>SPMAMTERLKVMTIFGTRPEAIKMAPLVLELQKHPEKIESIVTVTAQHRQMLDQVLSIFGITPDFDLNIMKDRQTLIDITTRGLEGLDKVMKEAKPDIVLVHGDTTTTFIASLAAFYNQIPVGHVEAGLRTWDKYSPYPEEMNRQLTGVMADLHFSPTAKSATNLQKENKDESRIFITGNTAIDALKTTVKETYSHPVLEKLGNNRLVLMTAHRRENLGEPMRNMFRAIKRLVDKHEDVQVVYPVHMNPVVRETANDILGDYGRIHLIEPLDVIDFHNVAAR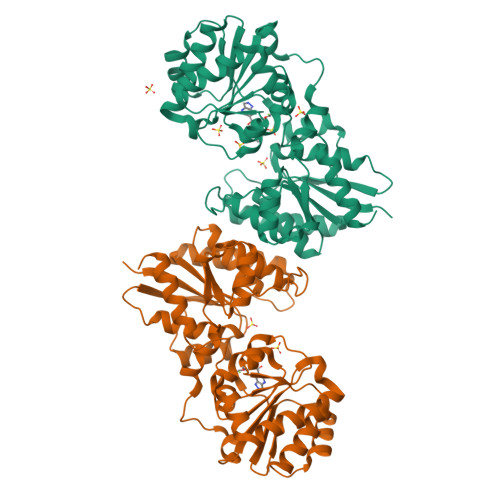SYLMLTDSGGVQEEAPSLGVPVLVLRDTTERPEGIEAGTLKLAGTDEETIFSLADELLSDKEAHDKMSKASNPYGDGRASERIVEAILKHFNK[2x]> SNAMEYYIVDSFATKLFKGNPAGVCVLDRRIPLELMQKIAEENNLPETAFVVKGKGNYELRWFTPKAEIDLCGHATLAAAYVISNFIDVNVKKI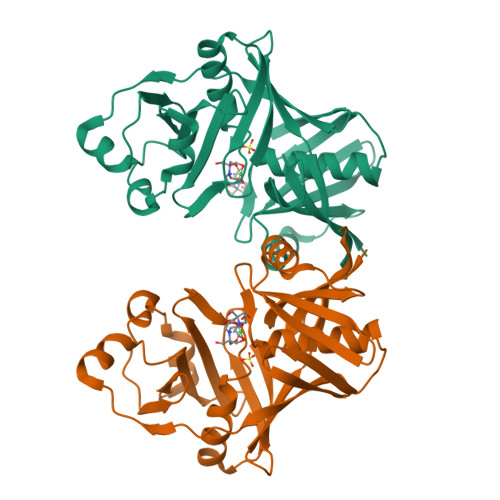DFFTQSGKLEVTRNGNLYEMIFPEIMPIEIELSPQQANLIGCVPSDVYSSRDLILLLNSEQEVINYKPNYAQLRKLTDWLGIIITAQGSNTDFVSRYFCPELDSEDPVTGSSHCNLIPYWSEKLGKHKMVAAQLSNRGGIIQCEVLKDNTVKISGEAVLFMQGTIKIDI>[4x]GTGAMIVKPMVRNNICLNAHPQGCKKGVEDQIEYTKKRITAEVKAGAKAPKNVLVLGCSNGYGLASRITAAFGYGAATIGVSFEKAGSETKYGTPGWYNNLAFDEAAKREGLYSVTIDGDAFSDEIKAQVIEEAKKKGIKFDLIVYSLASPVRTDPDTGIMHKSVLKPFGKTFTGKTVDPFTGEL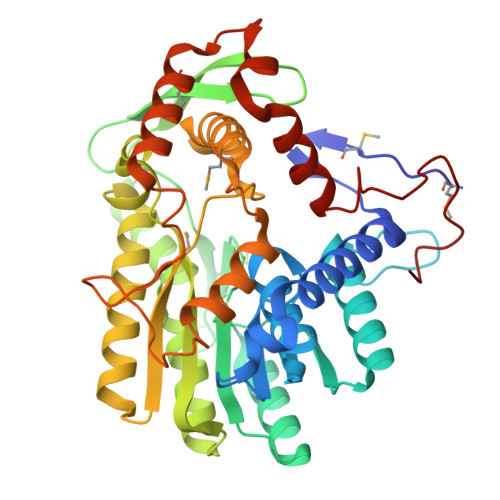KEISAEPANDEEAAATVKVMGGEDWERWIKQLSKEGLLEEGCITLAYSYIGPEATQALYRKGTIGKAKEHLEATAHRLNKENPSIRAFVSVNKGLVTRASAVIPVIPLYLASLFKVMKEKGNHEGCIEQITRLYAERLYRKDGTIPVDEENRIRIDDWELEEDVQKAVSALMEKVTGENAESLTDLAGYRHDFLASNGFDVEGINYEAEVERFDRI>[2x]MRGLSRRVQAMKPSATVAVNAKALELRRQGVDLVALTAGEPDFDTPEHVKEAARRALAQGKTKYAPPAGIPELREALAEKFRRENGLSVTPEETIVTVGGSQALFNLFQAILDPGDEVIVLSPYWVSYPEMVRFAGGVVVEVETLPEEGFVPDPERVRRAITPRTKALVVNSPNNPTGAVYPKEVLEALARL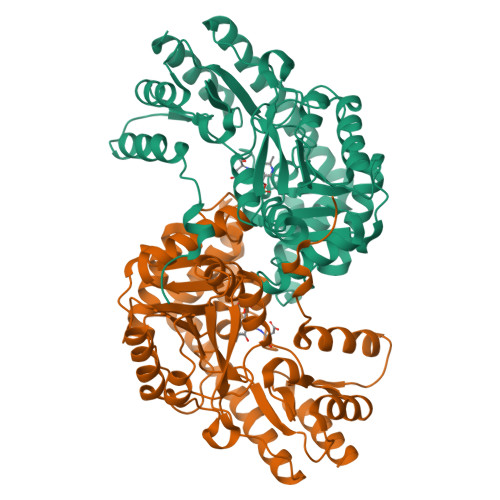AVEHDFYLVSDEIYEHLLYEGEHFSPGRVAPEHTLTVNGAAKAFAMTGWRIGYACGPKEVIKAMASVSRQSTTSPDTIAQWATLEALTNQEASRAFVEMAREAYRRRRDLLLEGLTALGLKAVRPSGAFYVLMDTSPIAPDEVRAAERLLEAGVAVVPGTDFAAFGHVRLSYATSEENLRKALERFARVLGRA> MVEATAQETDRPRFSFSIAAREGKARTGTIEMKRGVIRTPAFMPVGTAATVKALKPETVRATGADIILGNTYHLMLRPGAERIAKLGGLHSFMGWDRPILTDAGGYQVMSLSSLTKQSEEGVTFKSHLDGSRHMLSPERSI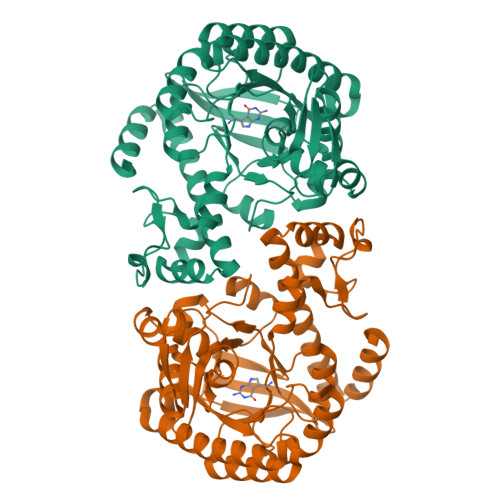EIQHLLGSDIVMAFDECTPYPATPSRAASSMERSMRWAKRSRDAFDSRKEQAENAALFGIQQGSVFENLRQQSADALAEIGFDGYAVGGLAVGEGQDEMFRVLDFSVPMLPDDKPHYLMGVGKPDDIVGAVERGIDMFDCVLPTRSGRNGQAFTWDGPINIRNARFSEDLKPLDSECHCAVCQKWSRAYIHHLIRAGEILGAMLMTEHNIAFYQQLMQKIRDSISEGRFSQFAQDFRARYFARNS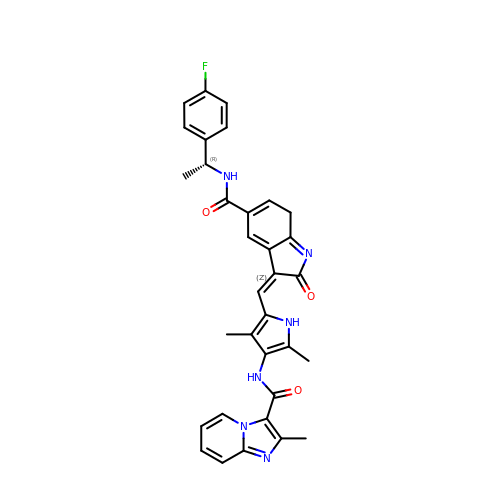(4S)-N-{5-[(Z)-(5-{[(1R)-1-(4-fluorophenyl)ethyl]carbamoyl}-2-oxo-2,7-dihydro-3H-indol-3-ylidene)methyl]-2,4-dimethyl-1H-pyrrol-3-yl}-2-methylimidazo[1,2-a]pyridine-3-carboxamide | C33 H29 F N6 O3 | WTFJOTYVTOMVRC-NAHYFOQLSA-N>[2x]MGLPPLLSLPSNSAPRSLGRVETPPEVVDFMVSLAEAPRGGRVLEPACAHGPFLRAFREAHGTAYRFVGVEIDPKALDLPPWAEGILADFLLWEPGEAFDLIL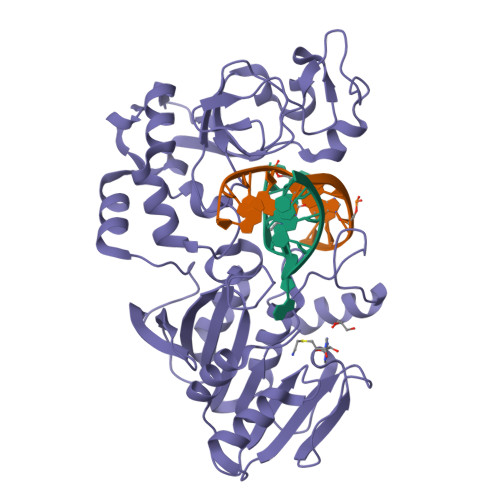GNPPYGIVGEASKYPIHVFKAVKDLYKKAFSTWKGKYNLYGAFLEKAVRLLKPGGVLVFVVPATWLVLEDFALLREFLAREGKTSVYYLGEVFPQKKVSAVVIRFQKSGKGLSLWDTQESESGFTPILWAEYPHWEGEIIRFETEETRKLEISGMPLGDLFHIRFAARSPEFKKHPAVRKEPGPGLVPVLTGRNLKPGWVDYEKNHSGLWMPKERAKELRDFYATPHLVVAHTKGTRVVAAWDERAYPWREEFHLLPKEGVRLDPSSLVQWLNSEAMQKHVRTLYRDFVPHLTLRMLERLPVRREYGFHTSPESARNF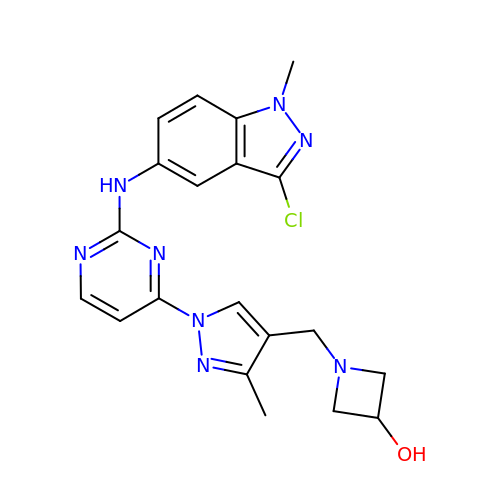1-[(1-{2-[(3-chloro-1-methyl-1H-indazol-5-yl)amino]pyrimidin-4-yl}-3-methyl-1H-pyrazol-4-yl)methyl]azetidin-3-ol | C20 H21 Cl N8 O | UCXIKENKSBLXSM-UHFFFAOYSA-N>[2x]MSDKEKPVRRSQAWFGRLDRDGFIYRSWMKNRGIPHDQFDGRPVIGICNTFSELTPCNSHFRTLAEQVKIGVWESGGFPLEFPVMSLGETMLRPTAMLFRNLASMDVEESIRGNPLDGVVLLMGCDKTTPSLMMGAASCDLPTIGVSGGPMLSGKFRGRELGSGTDVWKMSEEVRAGQMSQEEFFEAESCMHRSHGHCMTMGT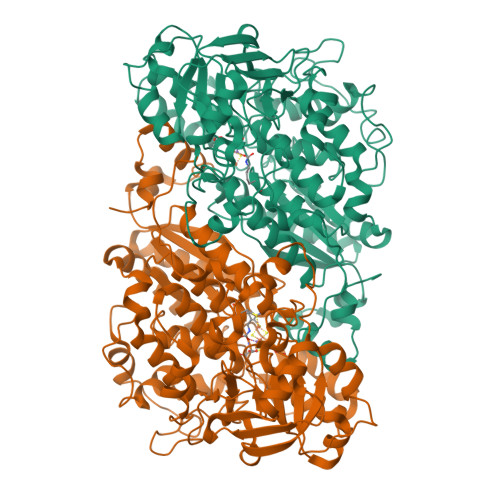ASTMASMVEALGMSLPGNAAIPAVDARRNLLARASGRRIVQMVKDDLVMSKILTRQAFENAIRVNAAIGGSTNAVIHLLAIAGRIGVDLTLADWDALGHKLPCLVDLQPSGTHLMEDFYYAGGVPAVIRELGDVIARDALTVNGQTLWDNCKDAPNWNREVIHAFNEPFKTEAGIAVLRGNLCPDGAVIKPSAATPALLKHKGRAVVFENSEHMHERMDDENLDVDENCVLVLKNCGPRGYPGMAEAGNMPLPPKILRKGITDMVRVSDARMSGTAYGTVVLHVAPEAAAGGPLALVQDGDIIELDVAARKLHLHVSDEELARRREAWQAPPAPMARGWVKLYVEHVQQANLGADLDFLRGKSGAGIPKDNH> MGSSHHHHHHMTCTLRDLNSLLEISSVRNDAQCCRCPAHNPSTAFAPTTKVRVSSDVRGIFALPVQKDHKPYNGLSPEHLETMKAVSLMLDAAGPKLEDGISKAKELLEERINPELMRDALGIYLTHSKDAQQRKIFPPPLKNHPFFSTKTRRPANVAGEICTADTLHGHALLSYWRDDYDLNDSHYYWHMVYRGAGGDNSKNVGDFDRHGEVFLYVHSQMVARYETESLCWSLPLVRPWNQYDDFLENGYAPISSLIEHYGGYPPFSTWYSIRNPDMPDTLNVTIPRARLEEWRDNIYAAIRKGQFETTSKDKPLVLTRDNCLNFVGGILDAQYPSLNKLLGGCSLDEERYGNLHNYGLGKFAEMAYRNKPGEKSPYGLTISNFGAPRDPCFWRWYKHLQYYGRLAATRYPQDITAHRAEVVLSNLVVRLQDRSSPHYLDGHITTFLGPPAVNFMESKAKLGHEPYEWNVQVKSCRRSPPSKENPQTLTLRLFIAAEDLMNDYHSWIEMDRATVQLTDESAITKVRLDTDSSVARKMGNYGEPDPRYASAVFRHGWPQNLMLPVGKVEGMPFVAFCIATDDGIPDPAPAPPFHHYHDPRGMGYPFNRAWTQLTEDSTGKASIRTIISNAELYPFITSTTFKIYRTTKFETKQIIQPTTVTWFNTIRGYFKDADRACMRSEYGYDLYNYDHVMLHADAILDATASKRMPLQMGKYTQDNPDPEHPLWTVKMCENFRAWLLNGCPKGTDP

Our experimental results clearly indicate that the hemocyanin-like protein AsqI is the cyclopenase, which is the enzyme in the viridicatin biosynthetic pathway that has eluded isolation for nearly four decades. Biochemical analysis reveals AsqI as a metalloprotein that requires zinc for its activity. In this reaction, the active-site zinc ion acts as a Lewis acid catalyst to activate the substrate epoxide and facilitate essentially an anti-Baldwin-type epoxide-opening 6-endo-tet cyclization. Subsequently, the conversion of a 6,7-bicyclic skeleton into a 6,6-bicyclic quinolone framework occurs upon elimination of 7 and the following keto–enol tautomerization results in the formation of the product.

Next, to establish the active-site architecture, the crystal structure of AsqI was determined. Based on the structure and the sequence homology of AsqI to hemocyanin, residues His176, His180, and His208 were identified to form the metal-binding site A in AsqI. However, the second tri-histidine metal-binding site B found in hemocyanins was formed by His346, Leu350, and Y387 in AsqI and no metal ion was observed there. While His346Ala mutation did not reduce the activity of AsqI, alanine mutation of each of the site-A histidine residues resulted in a nearly complete loss of activity, suggesting that the site-A metal plays a crucial role in substrate binding and catalysis. When AsqI was treated with ethylenediaminetetraacetic acid, it completely lost its cyclopenase activity. However, re-introduction of different metal ions (Fe2+, Fe3+, Co2+, Mn2+, Ni2+, Cu2+, and Zn2+) led to a varying degree of recovery of the activity, with zinc ion achieving the most outstanding recovery. Supplementing the reaction mixture with 30 µM ZnCl2 doubled kcat to 16.0 ± 0.30 min–1 but had a little effect on Km, which was 0.066 ± 0.0052 mM, indicating the important catalytic role the metal ion plays. To account for the role of zinc and the enzyme in the reaction of 5, we also optimized the structure of 5 in complex with Zn2+ and two imidazole molecules, which model the two histidine side chain groups identified experimentally as the metal ligands. The structure shows that the metal ion is coordinated to the imidazole molecules and the epoxide and C2 amide oxygen atoms of the substrate in a tetrahedral arrangement as frequently observed in zinc-complexed protein structures.>QGAMAMGVRNHRLLLLRHGETAWSTLGRHTGGTEVELTDTGRTQAELAGQLLGELELDDPIVICSPRRRTLDTAKLAGLTVNEVTGLLAEWDYGSYEGLTTPQIRESEPDWLVWTHGCPAGESVAQVNDRADSAVALALEHMSSRDVLFVSHGHFSRAVITRWVQLPLAEGSRFAMPTASIGI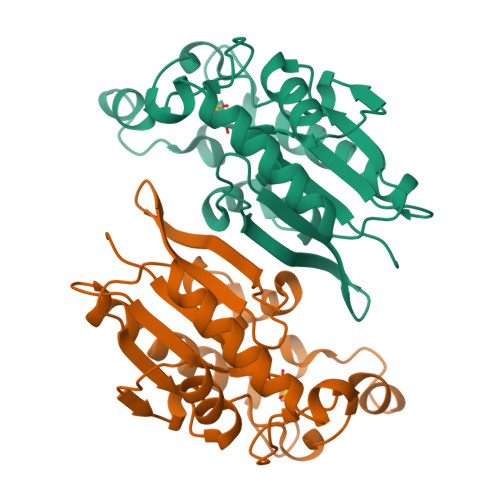CGFEHGVRQLAVLGLTGHPQPIAAG[2x]>GPMQQANLGDGVATARLLSRSDWGARLPKSVEHFQGPAPYVIIHHSYMPAVCYSTPDCMKSMRDMQDFHQLERGWNDIGFSFGIGGDGMIYTGRGFNVIGAHAPKYNDKSVGIVLIGDWRTELPPKQMLDAAKNLIAFGVFKGYIDPAYKLLGHRQVRDTECPGGRLFAEISSWPHFTHINDTEGVSSTTAPVVPHVHPQAAAPQKPHQSPPAAPKV[2x]

Drosophila PGRP-LB belongs to the amidase PGRPs and downregulates the immune deficiency (IMD) pathway by cleaving meso-2,6-diaminopimelic (meso-DAP or DAP)-type PGN. The structure of the PGRP domain comprises three α-helices and one central β-sheet composed of six β-strands, similar to the bacteriophage T7 lysozyme, a zinc-dependent amidase. The main difference between amidase and non-catalytic PGRPs is the presence of Zn2+ in only amidase PGRPs, which is coordinated by two histidines and one cysteine. We generated mutants to characterize the amidase reaction mechanism and solved the X-ray structures of wild-type Drosophila PGRP-LBPA/PC and its mutants in apo form or complexed to TCT.

The analysis of these results, including the first structure of a catalytic PGRP associated with TCT, highlighted the dynamic role of the residue Y78 in the amidase activity. In this structure elucidated to 1.80 Å resolution, the ligand is buried in a mostly positively charged pocket. Whereas the tetra-peptide is well defined, the carbohydrate moiety of TCT is not visible in the electron density. The absence of the electron density for the carbohydrate moiety of the TCT in the PGRP-LBPA/PC complexed structure is most probably due to its high flexibility. There are two possible pockets that can accept the sugar moiety of the ligand (annotated P1 and P2 in Figure 3A). The second pocket (P2) could accommodate the sugar moiety of the TCT. The specificity of the PGRP-LBPA/PC to the PGN is ensured by the recognition of the meso-DAP residue, interacting via hydrogen bonds with R92. The structure obtained here also shows another interesting interaction with a fourth coordination of Zn2+ made with the oxygen from the amide group of the TCT, which highlights the important role of Zn2+ in the enzymatic reaction. This interaction would increase the electrophilic character of the carbonyl group of the amide function where the amidase activity is occurring. By comparing the apo and complexed PGRP-LBPA/PC_Y78F structures, the C-terminal symmetry-related molecule is filling the binding pocket of the peptide moiety from the PGN attesting the non-physiological nature of this interaction.>[2x]MEYKSSPKRPYLLRAYYDWLVDNSFTPYLVVDATYLGVNVPVEYVKDGQIVLNLSASATGNLQLTNDFIQFNARFKGVSRELYIPMGAALAIYARENGDGVMFEPE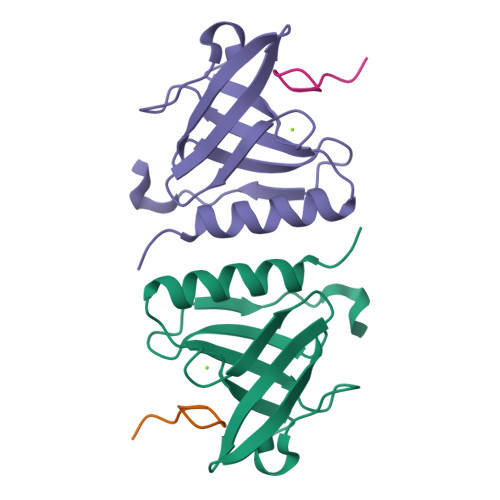EIYDE;>[2x]GRHGAANDENY> MEEKVESTTTPDGPCVVSVQETEKWMEEAMRMAKEALENIEVPVGCLMVYNNEVVGKGRNEVNQTKNATRHAEMVAIDQVLDWCHQHGQSPSTVFEHTVLYVTVEPCIMCAAALRLMKIPLVVYGCQNERFGGCGSVLNIASADLPNTGRPFQCIPGYRAEEAVELLKTFYKQENPNAPKSKVRKKDCQKS;> MEPTSGFAEQPGPVKAESEEQEPAQWQALPVLSEQQSGAVELILAYAAPVLDKRQTSRLLREVSAVYPLPAQPHLKRVRPSRSAGGAQSSDLLLCLAGPSAGPRSLAELLPRPAVDPRGLGTPFLVPLPARPPLTRSQFEEARAHWPTSFHEDKQVTSALAGQLFSTQERAAMQTHMERAVCAAQRAAAQGLRAVGAVVVDPASDRVLATGHDCSSVASPLLHAVMVCIDLVAQGQGEDSLPYVCTGYDLYVTREPCVMCAMALVHARIQRVFYGAPSPDGALGTLFRVHA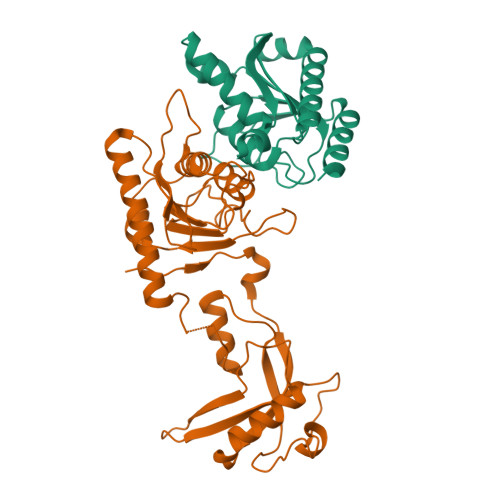RPDLNHRFQVFRGILEDQCRQLDPDP Tropomodulins (Tmods) constitute a conserved family of four isoforms that work in conjunction with one of several tropomyosin (TM) isoforms to cap the pointed end of actin filaments in cytoskeletal structures characterized by their uniform distribution of the lengths of actin filaments. Leiomodins (Lmods) are related to Tmods, and constitute a subfamily of three isoforms: Lmod1, expressed preferentially in differentiated smooth muscle cells; and Lmod2 and Lmod3, expressed more abundantly in skeletal and cardiac muscles89101112. Lmods are distinguished from Tmods by the presence of a C-terminal extension, featuring a proline-rich region and a WH2 domain. We show that ABS2, and not the C-terminal extension, is the main factor distinguishing Lmods and Tmods as filament nucleators and pointed-end-capping proteins, respectively.

Similar results were obtained with Lmod1, although in this case removing the N-terminal region had nearly no effect on the nucleation activity, and the isolated ABS2 had even stronger activity than that of Lmod2. The structure of Lmod1ABS2, the strongest nucleator among the naturally occurring ABS2s analysed here, was determined at 1.54 Å resolution, and shows residues Ala-314 to Gln-486. The structure superimposes well with that of Tmod1ABS2, with a root mean squared deviation (r.m.s.d.) of 0.57 Å for 131 equivalent Cα atoms. The major differences occur at the N and C termini of the domain, consistent with the lower sequence conservation observed within these areas. The C-terminal helix is rotated ∼4° compared with Tmod1ABS2. However, this difference does not necessarily correlate to function, since the C-terminal helix is generally flexible and changes conformation when bound to actin7. The differences at the N terminus appear to be more important. Indeed, the loop of Tmod1 implicated in pointed-end capping (Tyr-170 to Val-183) is missing in Lmods, and the corresponding region of Lmod1 visualized in the electron density map (Ala-314 to Phe-318) is oriented in the opposite direction to that of Tmod1ABS2 in the unbound as well as the actin-bound structures. First, in Lmod ABS2 lacks the N-terminal region that in Tmod interacts with the DNase I-binding loop at the pointed end of the second actin subunit of the filament.

> PTKPSEGPAKVEEEAAPSIFDEPLERVKNNDPEMTEVNVNNSDCITNEILVRFTEALEFNTVVKLFALANTRADDHVAFAIAIMLKANKTITSLNLDSNHITGKGILAIFRALLQNNTLTELRFHNQRHICGGKTEMEIAKLLKENTTLLKLGYHFELAGPRMTVTNLLSRNMDKQRQKRLQEQRQAQ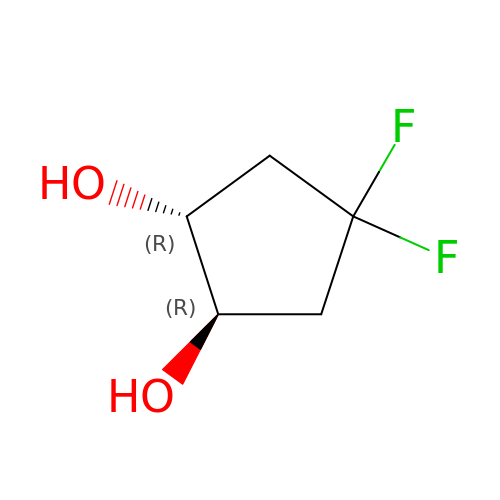(1~{R},2~{R})-4,4-bis(fluoranyl)cyclopentane-1,2-diol | C5 H8 F2 O2 | RQJNPJXCMOLSSC-QWWZWVQMSA-N THIOPHENE-2-CARBOXYLIC ACID | 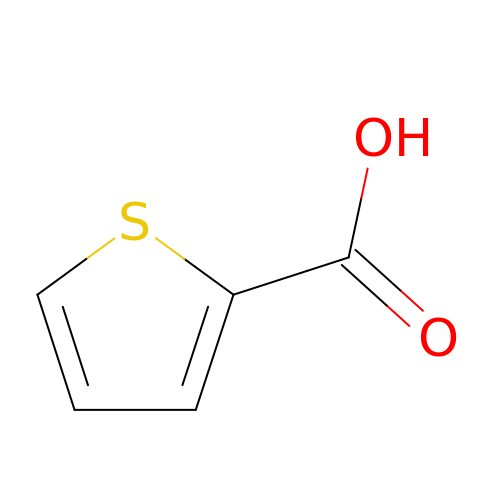C5 H4 O2 S | QERYCTSHXKAMIS-UHFFFAOYSA-N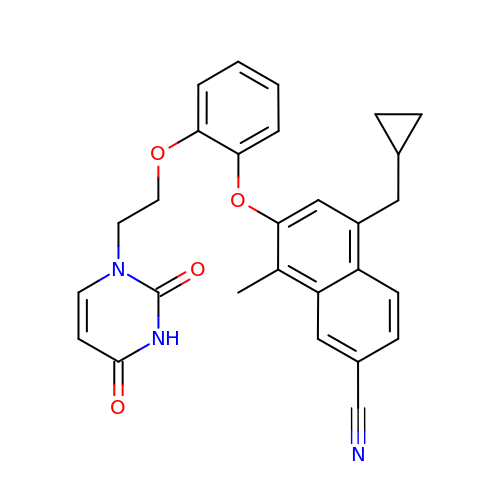5-(cyclopropylmethyl)-7-{2-[2-(2,4-dioxo-3,4-dihydropyrimidin-1(2H)-yl)ethoxy]phenoxy}-8-methylnaphthalene-2-carbonitrile | C28 H25 N3 O4 | VAFJQCGXOLTBQY-UHFFFAOYSA-N> GYFSAADVYVPDEWEVAREKITMSRELGQGSFGMVYEGVAKGVVKDEPETRVAIKTVNEAASMRERIEFLNEASVMKEFNCHHVVRLLGVVSQGQPTLVIMELMTRGDLKSYLRSLRPEMENNPVLAPPSLSKMIQMAGEIADGMAYLNANKFVHRDLAARNCMVAEDFTVKIGDFGMTRDIYETDYYRKGGKGLLPVRWMSPESLKDGVFTTYSD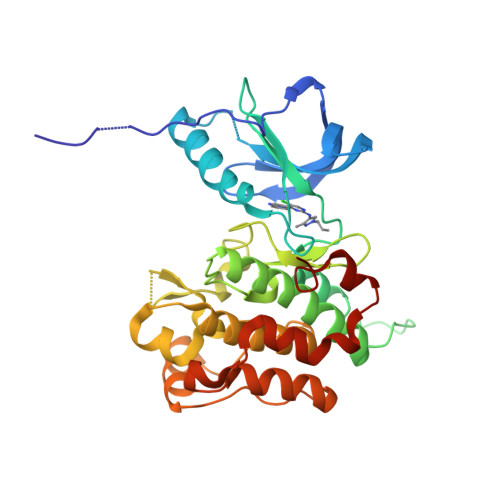VWSFGVVLWEIATLAEQPYQGLSNEQVLRFVMEGGLLDKPDNCPDMLFELMRMCWQYNPKMRPSFLEIISSIKEEMEPGFREVSFYYSEENK> MRGSHHHHHHGSWETEERPRTREEESHFYAGGQVYPGEASRVSVADHSLHLSKAKISKPAPYWEGTAVIDGEFKELKLTDYRGKYLVFFFYPLDFTFVSPTEIIAFGDRLEEFRSINTEVVACSVDSQFEHLAWINTPRRQGGLGPIRIPLLSDLTHQISKDYGVYLEDSGHTLRGLFIIDDKGILRQITLNDLPVGRSVDETLRLVQAFQYTDKHGEVCPAGWKPGSETIIPDPAGKLKYF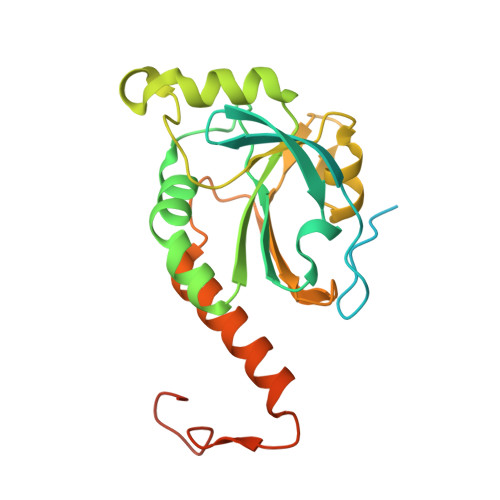DKLN>MSLPTTIQAISAEAINLPLTEPFAIASGAQAVAAN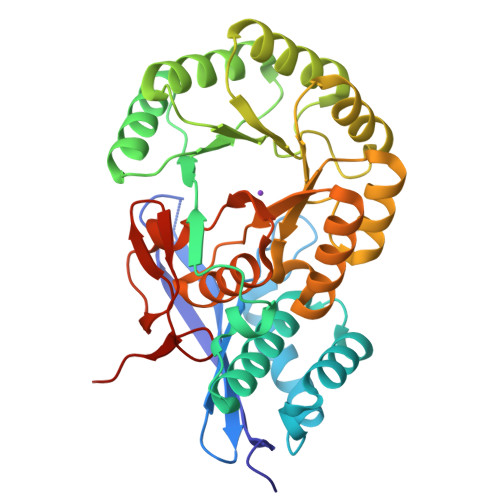VLVKVQLADGTLGLGEAAPFPAVSGETQTGTSAAIERLQSHLLGADVRGWRKLAAMLDHAEHEAAAARCGLEMAMLDALTRHYHMPLHVFFGGVSKQLETDMTITAGDEVHAAASAKAILARGIKSIKVKTAGVDVAYDLARLRAIHQAAPTAPLIVDGNCGYDVERALAFCAACKAESIPMVLFEQPLPREDWAGMAQVTAQSGFAVAADESARSAHDVLRIAREGTASVINIKLMKAGVAEGLKMIAIAQAAGLGLMIGGMVESILAMSFSANLAAGNGGFDFIDLDTPLFIAEHPFIGGFAQTGGTLQLADVAGHGVNLEGHHHHHH[4x]> GSNNVLPTWSLDSNGEMRSRLSLSEVLDSGDLMKFAVDKTGCQFLEKAVKGSLTSYQKFQLFEQVIGRKDDFLKLSTNIFGNYLVQSVIGISLATNDDGYTKRQEKLKNFISSQMTDMCLDKFACRVIQSSLQNMDLSLACKLVQALPRDARLIAICVDQNANHVIQKVVAVIPLKNWEFIVDFVATPEHLRQICSDKYGCRVVQTIIEKLTADSMNVDLTSAAQNLRERALQRLMTSVTNRCQELATNEYANYIIQHIVSNDDLAVYRECIIEKCLMRNLLSLSQEK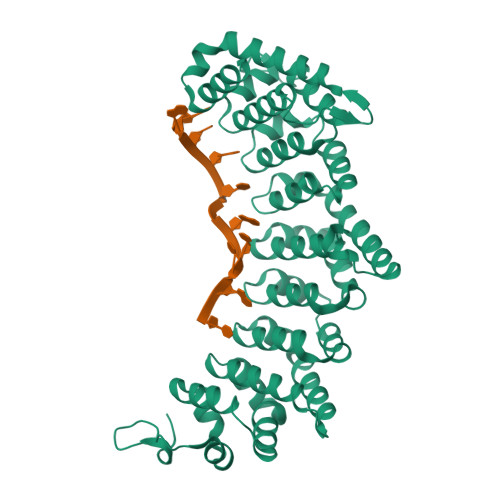FASHVVEKAFLHAPLELLAEMMDEIFDGYIPHPDTGKDALDIMMFHQFGNYVVQCMLTICCDAVSGRRQTKEGGYDHAISFQDWLKKLHSRVTKERHRLSRFSSGKKMIETLANLRSTHPIYELQ Vps33 regulates fusion in the endo-lysosomal membrane system as a stable subunit within two large multisubunit tethering complexes, HOPS (homotypic fusion and vacuolar protein sorting) and CORVET (class C core vacuole/endosome tethering). Vps33 shares the overall shape and topology observed for previously reported SM protein structures. Following the nomenclature introduced by Misura et al., Vps33 contains three domains: domain 1 (residues 1–138; red), domain 2 (residues 139–248 and 502–667; green), and domain 3 (residues 249–501; blue), with domain 3 further subdivided into 3a (residues 249–380) and 3b (residues 381–501). The C. thermophilum Vps33 and Vps16CTD–Vps33 structures provide a first detailed view of an SM protein from the Vps33 family and of its recruitment into a multisubunit tethering complex.

As an alternative, we co-expressed and crystallized Vps33 with a C-terminal fragment of Vps16 (Vps16CTD; residues 505–834). The structure of the C. thermophilum Vps16CTD–Vps33 complex was determined by molecular replacement using C. thermophilum Vps33 as a search model and was refined to 2.6 Å resolution. Vps16CTD contains an irregular α-solenoid made up of 17 α-helices arranged in a manner similar to HEAT repeat proteins. Vps16CTD binds to the upper surface of the Vps33 arch, opposite the large cleft between Vps33 domains 1 and 3. In so doing, it interacts with all three domains of Vps33, burying about 4800 Å2 of accessible surface area in the interface. The N-terminal portion of Vps16CTD lies in the groove between domains 1 and 2 of Vps33; the majority of the Vps16CTD–Vps33 contacts in this region involve polar rather than hydrophobic residues. The contact surface with domain 3b entails a mixture of polar and non-polar interactions involving Vps16 helices α8-α13; the long α10 helix packs especially extensively against Vps33. Interestingly, three residues near the C-terminus of Vps33 (residues 655–657), which are disordered in the uncomplexed protein, adopt a well-ordered conformation in the Vps16CTD–Vps33 complex. Nonetheless, despite the extensive interaction between Vps33 and Vps16CTD, the backbone conformation of Vps33 is almost identical to that observed for the uncomplexed protein (root-mean-squared deviation <0.6 Å). In the Vsp16CTD–Vps33 structure, no interpretable electron density was observed for this region of Vps33 (residues 334–356), suggesting that in the absence of crystallographic contacts the tip is flexible.

> GSMAPRAGFDAEQVRDKARKDLLHLLEGVRGKKNLVIEKDLAGPLGVIVKASTLRDYGVDNFFFLENKNTGTSQRNIVFIARGESVRNAHAIAAQIKRIQRESQTSHDFHIFWVPRRTLFSDKVLEEAGVLGDANISELPLYFFPLERDVLSLELNDSFRDLYLAKDPTPVFLLSRALMGIQKKHGLFPRIIGKGENAKRVADLLSRMRQELLAGEEAGESDRAGLSPSTTIESVIIIDREVDFVTPLLTQLTYEGLIDEYFGIQNNQTDVDAVIVGAPAQSAASTSTAVPTNSSQSRKRKIQLDGSDSLYSQLRDANFAIVGSLLNTVARRLKSDYESRHNTKTTAELKEFVKKLPGYQAEQQSLKIHSNIAEEIINYTRTEIFNKLLEVQQNLAAGADPSSQFDSIEELVARDTPLPQVLRLLCLYSCISGGIKTKELDHFRRLVLQGYGHQHLLTLHNLERLQMFLSKSSPLASMITMSGSSGGPDQKTNYTYLRKQLRLIVDEVNEQDPNDIAYVYSGYAPLSIRLVQCVLQKQYLLSITKGSGTVIAAGPVAGGGAQGWKGFEEIVKHARGPTFDEIQKGEDKAVKARALLSGSSGDKKTVFVVFVGGITFTEIAALRFIAKQEEARRNIVICTTSIINGNRMMNAAIETATFEKTTVTTAAAQ;> MGSSFEVIARTAYEEGRTRLATELLNHEPRAGRQVPLLLSMEEDELALDKAIESGDTDLIYFVIHQLRRKLPLASFFRVVSSRPTASAMVEALARNSDGDGNEDTALLKDLYYQDDRRLDGASVFIREALQQPETRTASDKLDLAANLLQGNQKEHVFELGALKEAKMLLRMQETFERDLTDSFVGLSVNQTMFKLIKLGYHGRAKKIQSEFKVPERVAWWIRLQALVAKRDWNEIEEISRQRKSPIGWEPFFNQVLQAGNPRLAATFIPKCTNLEPGQTITMYEKCGMRVKAAEEAVRLKDTEAWNRLLEAAGRNTAEGREIERLGATVFKK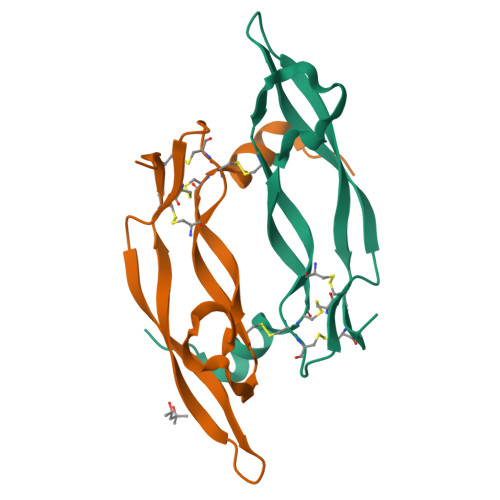>[2x]HQRKVVSWIDVYTRATCQPREVVVPLTVELMGTVAKQLVPSCVTVQRCGGCCPDDGLECVPTGQHQVRMQILMIRYPSSQLGEMSLEEHSQCECRPKKK>GRSRLLEDFRNNRYPNLQLREIAGHIMEFSQDQHGSRFIQLKLERATPAERQLVFNEILQAAYQLMVDVFGNYVIQKFFEFGSLEQKLALAERIRGHVLSLALQMYGCRVIQKALEFIPSDQQNEMVRELDGHVLKCVKDQNGNHVVQKCIECVQPQSLQFIIDAFKGQVFALSTHPYGCRVIQRILEHCLPDQTLPILEELHQHTEQLVQDQYGNYVIQHVLEHGRPEDKSKIVAEIRGNVLVLSQHKFASNVVEKCVTHASRTERAVLIDEVCTMNDGPHSALYTMMKDQYANYVVQKMIDVAEPGQRKIVMHKIRPHIATLRKYTYGK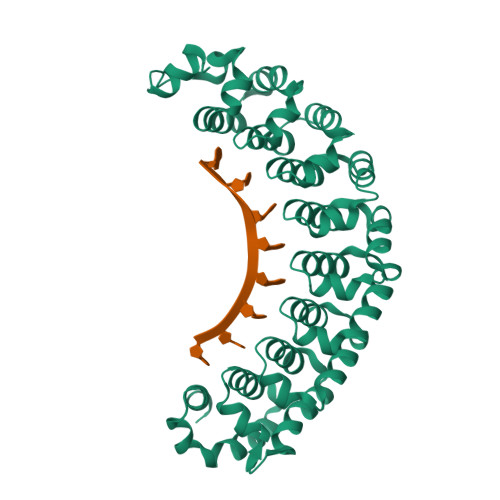HILAKLEKYYMKNGVDLG[2x]> SIRNRRPELLPNDCGYQVEADKILNGDDTVPEEFPWTAMIGYKNSSNFEQFACGGSLINNRYIVTA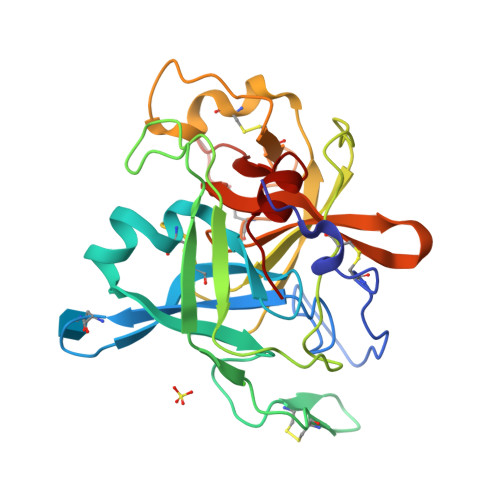AHCVAGRVLRVVGALNKVRLGEWNTATDPDCYGAVRVCVPDKPIDLGIEETIQHPDYVDGSKDRYHDIALIRLNRQVEFTNYIRPVCLPQPNEEVQVGQRLTVVGWGRTETGQYSTIKQKLAVPVVHAEQCAKTFGAAGVRVRSSQLCAGGEKAKDSCGGDSGGPLLAERANQQFFLEGLVSFGATCGTEGWPGIYTKVGKYRDWIEGNIRP>[2x]GAMVAKPFQRLIDLIGHMTLSDFTRFPNLKEAISWPLGEPSLAFFDLS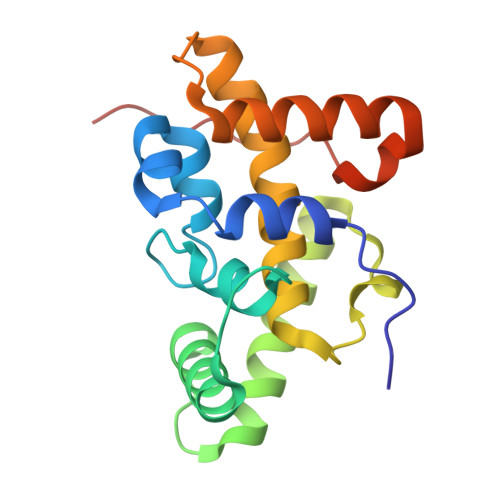STRVHRNDDIRRDQIATLAMRSCKITNDLEDSFVGLHRMIATEAILRGIDLCLLPGFDLMYEVAHVQCVRLLQAAKEDISNAVVPNSALIVLMEESLMLRSSLPSMMGRNNWIPVIPPIPDV> MSLKYKNLFFDLDDTIWAFSRNARDTFEEVYQKYSFDRYFDSFDHYYTLYQRRNTELWLEYGEGKVTKEELNR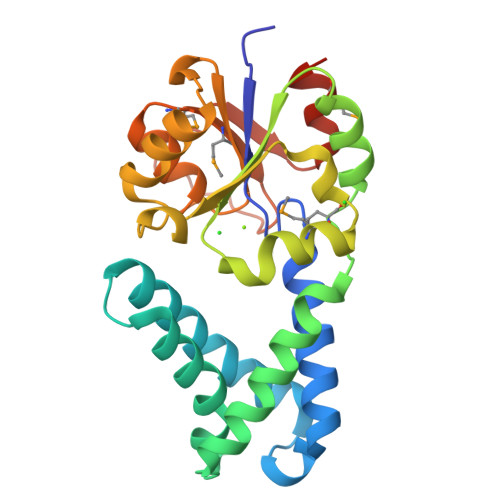QRFFYPLQAVGVEDEALAERFSEDFFAIIPTKSGLMPHAKEVLEYLAPQYNLYILSNGFRELQSRKMRSAGVDRYFKKIILSEDLGVLKPRPEIFHFALSATQSELRESLMIGDSWEADITGAHGVGMHQAFYNVTERTVFPFQPTYHIHSLKELMNLLEGHHHHHH N-((3S,4S)-5-[(4-BROMOBENZYL)OXY]-3-HYDROXY-4-{[N-(PYRIDIN-2-YLCARBONYL)-L-VALYL]AMINO}PENTANOYL)-L-ALANYL-L-LEUCINAMIDE | C32 H45 Br N6 O7 | 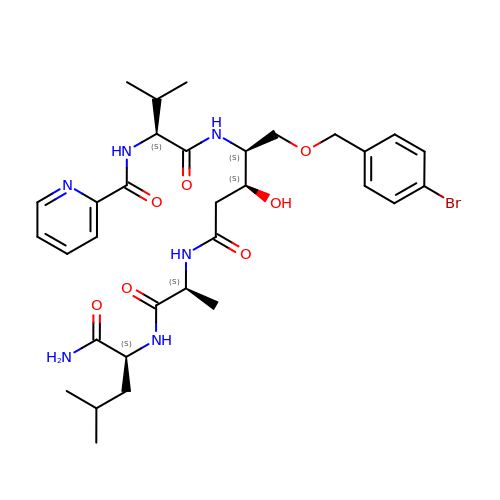QXHNYZQKWOKULQ-QPGFMSSHSA-N> GSHMGGPIKIIDP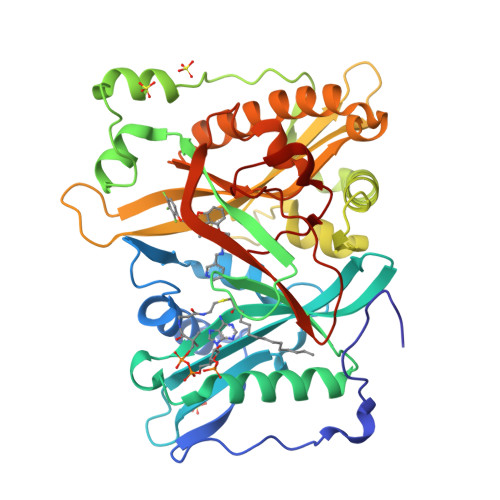EKVSKEPDALLEGFEWATLDLTNETELQELWDLLTYHYVEDDNAMFRFRYSQSFLHWALMSPGWKKEWHVGVRATKSRKLVASICGVPTEINVRNQKLKVVEINFLCIHKKLRSKRLTPVLIKEITRRCYLNGIYQAIYTAGVVLPTPVSSCRYYHRPLDWLKLYEVGFSPLPAGSTKARQITKNHLPSTTSTPGLRPMEPKDIDTVHDLLQRYLSRFALNQAFTREEVDHWLVHKPETVKEQVVWAYVVEDPETHKITDFFSFYNLESTVIQNPKHDNVRAAYLYYYATETAFTNNMKALKERLLMLMNDALILAKKAHFDVFNALTLHDNPLFLEQLKFGAGDGQLHFYLYNYRTAPVPGGVNEKNLPDEKRMGGVGIVML> ASPRELTQNPLKKIFMPYSNGRPALHASQRGVCMTNCPTLIVMVGLPARGKTYISKKLTRYLNFIGVPTREFNVGQYRRDMVKTYKSFEFFLPDNEEGLKIRKQCALAALNDVRKFLSEEGGHVAVFDATNTTRERRAMIFNFGEQNGYKTFFVESICVDPEVIAANIVQVKLGSPDYVNRDSDEATEDFMRRIECYENSYESLDEEQDRDLSYIKIMDVGQSYVVNRVADHIQSRIVYYLMNIHVTPRSIYLCRHGESELNLKGRIGGDPGLSPRGREFSKHLAQFISDQNIKD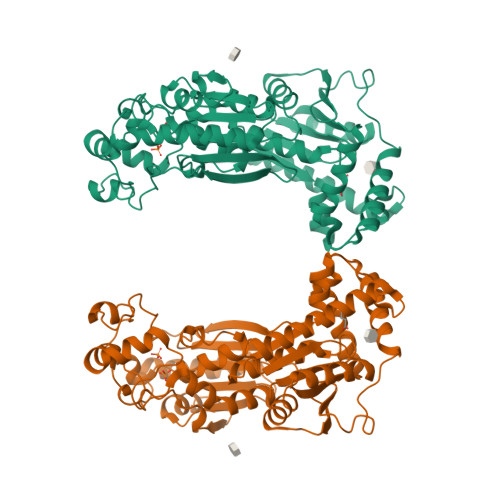LKVFTSQMKRTIQTAEALSVPYEQFKVLNEIDAGVCEEMTYEEIQDHYPLEFALRDQDKYRYRYPKGESYEDLVQRLEPVIMELERQENVLVICHQAVMRCLLAYFLDKAAEELPYLKCPLHTVLKLTPVAYGCKVESIFLNVAAVNTHRDRPQNVDISRPSEEALVTVPAHQ>GGDSRELIARYQILLAELAAIRADIAAERTGDPYVRKLARELKRLAQEAAEEVKRDPSSSDVNMALLLILLMIELAVRALEAAERTGDPEVRELAAELVWLAVEAAEEVQRNPSSSDVWLALHLIMLAIWAAVAALEAAERTGDPEVRELARELVRLAVEAAEEVQRNPSSKEVYMALLLILIAILEAVLSLLRAERSGDPEKREKARERVREAVERAEEVQR[2x]

To investigate the photophysics of special pairs independently of the complexities of native photosynthetic proteins, and as a first step toward creating synthetic photosystems for new energy conversion technologies, we designed C2-symmetric proteins that hold two chlorophyll molecules in closely juxtaposed arrangements. For Chl dimer protein scaffolds, we chose hyperstable C2-symmetric repeat protein dimers containing symmetric pockets with tunable sizes and geometries. In this dimeric repeat protein architecture, the hydrophobic core is independent of the small molecule-binding site, enabling full customization for binding with little impact on the overall protein structure. We describe de novo-designed proteins that hold Chl dimers in precisely defined, closely juxtaposed geometries.

The X-ray crystal structure of SP1 was solved in the ZnPPaM-bound state to 2.0 Å resolution, revealing a special pair geometry closely matching that of purple photosynthetic bacteria. The r.m.s.d. between the ZnPPaM dimer in the SP1 crystal structure and its design model is 0.25 Å. Hydrogen bonds to the ring E ketone group, which has been shown to be important for modulating special pair redox potentials, form with Gln10 in both ZnPPaM molecules, in agreement with the design model. We obtained crystal structures of two holo-state designs: the first, SP1, reproduces the binding geometry of the native purple bacterial reaction center special pair with sub-Ångstrom precision, and the second, SP2, has a distinct geometry with the Chl molecules closer together. Calculations on the SP1−ZnPPaM dimer crystal structure yielded a lower excitonic coupling of 87 cm−1. Experimental low-temperature spectra of SP1−ZnPPaM in 40% glycerol showed only a modest broadening of the SP1−ZnPPaM dimer fluorescence emission band compared with the monomer, consistent with weaker excitonic coupling. SP1 exhibits weaker excitonic coupling than SP2 and the BChl special pair of purple photosynthetic bacteria, despite its close structural similarity to the latter. We found that the signs of the CD Cotton effects predicted from the crystal structures of SP1 and SP2 were consistent with the experimental signs in the Qy region.>[2x]AATYAQTLQNIPETNVTTLDNGLRVASEESSQPTCTVGVWIGAGSRYENEKNNGAGYFVEHLAFKGTKKRPCAAFEKEVESMGAHFNGYTSREQTAFYIKALSKDMPKVVELLADVVQNCALEESQIEKERGVILQELKEMDNDMTNVTFDYLHATAFQGTALARTVEGTTENIKHLTRADLASYIDTHFKAPRMVLAAAGGISHKELVDAARQHFSGVSFTYKEDAVPILPRCRFTGSEIRARDDALPVAHVALAVEGPGWADPDNVVLHVANAIIGRYDRTFGGGKHLSSRLAALAVEHKLCHSFQTFNTSYSDTGLFGFHFVADPLSIDDMMFCAQGEWMRLCTSTTESEVKRAKNHLRSAMVAQLDGTTPVCETIGSHLLNYGRRISLEEWDSRISAVDARMVRDVCSKYIYDKCPALAAVGPIEQLLDYNRIRSGMYWIRF;>SLKVAPKVAVSAAAERVKLCPGAEDLEITKLPNGLIIASLENFSPASRIGVFIKAGSRYETTANLGTAHLLRLASPLTTKGASSFRITRGIEAVGGSLSVYSTREKMTYCVECLRDHVDTVMEYLLNVTTAPEFRPWEVTDLQPQLKVDKAVAFQSPQVGVLENLHAAAYKTALANPLYCPDYRIGKITSEQLHHFVQNNFTSARMALVGIGVKHSDLKQVAEQFLNIRSGAGTSSAKATYWGGEIREQNGHSLVHAAVVTEGAAVGSAEANAFSVLQHVLGAGPLIKRGSSVTSKLYQGVAKATTQPFDASAFNVNYSDSGLFGFYTISQAAHAGEVIRAAMNQLKAAAQGGVTEEDVTKAKNQLKATYLMSVETAQGLLNEIGSEALLSGTHTAPSVVAQKIDSVTSADVVNAAKKFVSGKKSMAASGDLGSTPFLDEL[2x];>MAPNIRKSHPLLKMINNSLIDLPAPSNISAWWNFGSLLAVCLMTQILTGLLLAMHYTADTSLAFSSVAHTCRNVQYGWLIRNLHANGASFFFICIFLHIGRGLYYGSYLYKETWNTGVILLLTLMATAFVGYVLPWGQMSFWGATVITNLFSAIPYIGHTLVEWAWGGFSVDNPTLTRFFALHFLLPFAIAGITIIHLTFLHESGSNNPLGISSDSDKIPFHPYYSFKDILGLTLMLTPFLTLALFSPNLLGDPENFTPANPLVTPPHIKPEWYFLFAYAILRSIPNKLGGVLALAASVLILFLIPFLHKSKQRTMTFRPLSQTLFWLLVANLLILTWIGSQPVEHPFIIIGQMASLSYFTILLILFPTIGTLE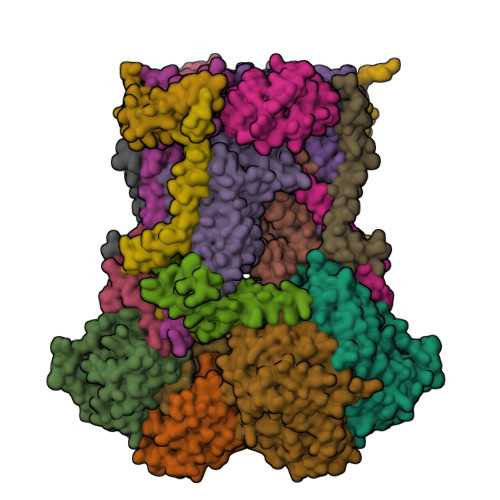NKMLNY[2x];>GELELHPPAFPWSHGGPLSALDHSSVRRGFQVYKQVCSACHSMDYVAFRNLIGVTHTEAEAKALAEEVEVQDGPDENGELFMRPGKISDYFPKPYPNPEAARAANNGALPPDLSYIVNARHGGEDYVFSLLTGYCDPPAGVVVREGLHYNPYFPGQAIGMAPPIYNEILEYDDGTPATMSQIAKDVCTFLRWAAEPEHDQRKRMGLKMLLISALLTSLLYYMKRHKWSVLKSRKMAYRPPK[2x];>[2x]VHNDVTVPDFSAYRREDVMDATTSSQTSSEDRKGFSYLVTATACVATAYAAKNVVTQFISSLSASADVLALSKIEIKLSDIPEGKNVAFKWRGKPLFVRHRTQAEINQEAEVDVSKLRDPQHDLDRVKKPEWVILVGVCTHLGCVPIANSGDFGGYYCPCHGSHYDASGRIRKGPAPYNLEVPTYQFVGDDLVVVG;>AARATVAGGGRLMDRIRKWYYNAAGFNKYGLMRDDTLYEDDDVKEALKRLPEDLYNERMFRIKRALDLSLKHRILPKEQWVKYEEDKPYLEPYLKEVIRERLEREAWNKK[2x];>GIHFGNLARVRHIITYSLSPFEQRAIPNIFSDALPNVWRRFSSQVFKVAPPFLGAYLLYSWGTQEFERLKRKNPADYENDQ[2x];>[2x]LRGSGEEEEEELVDPLTTIREHCEQTEKCVKARERLELCDARVSSRSHTEEQCTEELFDFLHARDHCVAHKLFNKLK;>ALLRQAYSALFRRTSTFALTVVLGAVLFERAFDQGADAIFEHLNEGKLWKHIKHKYEASEE[2x]> MADVLSVGVNLEAFSQAISAIQALRSSVSRVFDCLKDGMRNKETLEGREKAFIANFQDNLHSVNRDLNELERLSNLVGKPSENHPLHNSGLLSLDPVQDKTPLYSQLLQAYKWSNKLQYHAGLASGLLNQQSLKRSANQMGVSAKRRPKAQPTTLVLPPQYVDDVISRIDRMFPEMSIHLSRPNGTSAMLLVTLGKVLKVIVVMRSLFIDRTIVKGYNESVYTEDGKLDIWSKSSYQVFQKVTDHATTALLHYQLPQMPDVVVRSFMTWLR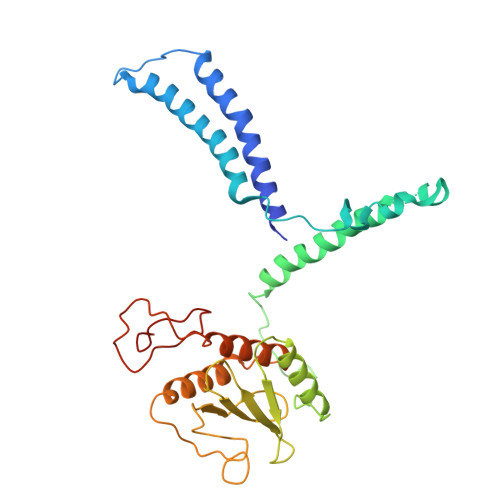SYIKLFQAPCQRCGKFLQDGLPPTWRDFRTLEAFHDTCRQ>MAETPNSDMSGATGGRSKRPKSNQDWWPSKLNLEILDQNARDVGPVEDDFDYAEEFQKLDLEAVKSDLEELMTSSQDWWPADYGHYGPLFIRMAWHSAGTYRTADGRGGAAGGRQRFAPINSWPDNANLDKARRLLLPIKQKYGQKISWADLMILAGNVAIESMGFKTFGYAGGREDAFEEDKAVNWGPEDEFETQERFDEPGEIQEGLGASVMGLIYVNPEGPDGNPDPEASAKNIRQTFDRMAMNDKETAALIAGGHTFGKVHGADDPEENLGPEPEAAPIEQQGLGWQNKNGNSKGGEMITSGIEGPWTQSPTEWDMGYINNLLDYEWEPEKGPGGAWQWAPKSEELKNSVPDAHDPDEKQTPMMLTTDIALKRDPDYREVMETFQENPMEFGMNFAKAWYKLTHLDMGPPERFLGPEVPDEEMIWQDPLPDADYDLIGDEEIAELKEEILDSDLSVSQLVKTAWASASTYRDSDKRGGANGARLRLEPQKNWEVNEPEQLETVLGTLENIQTEFNDSRSDG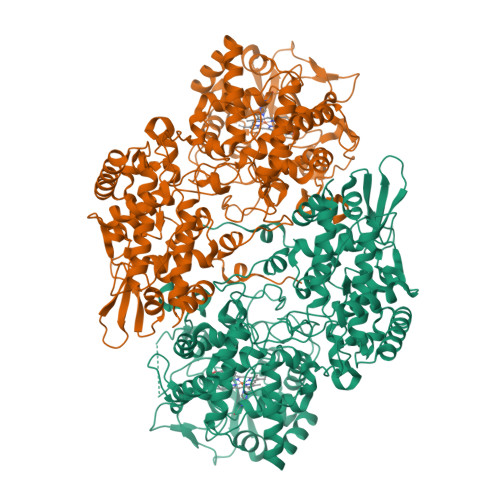TQVSLADLIVLGGNAAVEQAAANAGYDVEIPFEPGRVDAGPEHTDAPSFDALKPKVDGVRNYIQDDITRPAEEVLVDNADLLNLTASELTALIGGMRSIGANYQDTDLGVFTDEPETLTNDFFVNLLDMGTEWEPAADSEHRYKGLDRDTGEVKWEATRIDLIFGSNDRLRAISEVYGSADAEKKLVHDFVDTWSKVMKLDRFDLEHHHHHH[2x]(2R,3aS,5aR,5bS,9S,13S,14R,16aS,16bR)-9-ethyl-2,13-dihydroxy-14-methyl-2,3,3a,5a,5b,6,9,10,11,12,13,14,16a,16b-tetradecahydro-1H-as-indaceno[3,2-d]oxacyclododecine-7,15-dione | C24 H34 O5 | 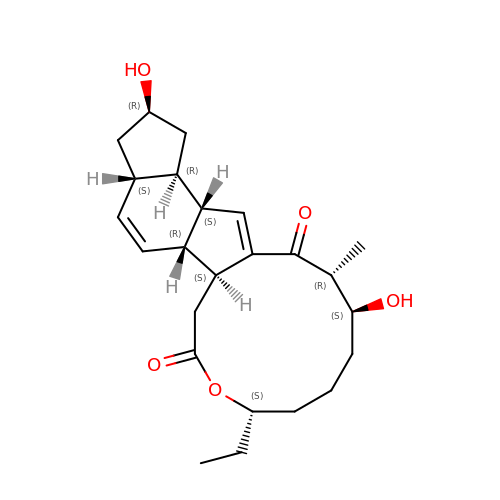DIHUILSVOGYVDG-MRAVEKNJSA-N> XSEAAAST;> WMDFX;>[2x]HGSPVDICTAKPRDIPMNPMCIYRSPEKKATEDEGSEQKIPEATNRRVWELSKANSRFATTFYQHLADSKNDNDNIFLSPLSISTAFAMTKLGACNDTLQQLMEVFKFDTISEKTSDQIHFFFAKLNCRLYRKANKSSKLVSANRLFGDKSLTFNETYQD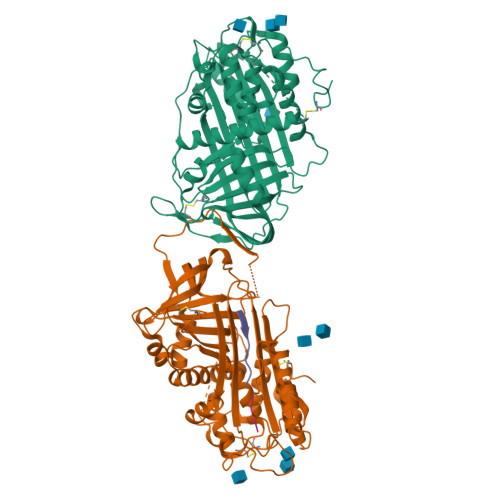ISELVYGAKLQPLDFKENAEQSRAAINKWVSNKTEGRITDVIPSEAINELTVLVLVNTIYFKGLWKSKFSPENTRKELFYKADGESCSASMMYQEGKFRYRRVAEGTQVLELPFKGDDITMVLILPKPEKSLAKVEKELTPEVLQEWLDELEEMMLVVHMPRFRIEDGFSLKEQLQDMGLVDLFSPEKSKLPGIVAEGRDDLYVSDAFHKAFLEVNEEGSEAAASTAVVIAGRSLNPNRVTFKANRPFLVFIREVPLNTIIFMGRVANPCVK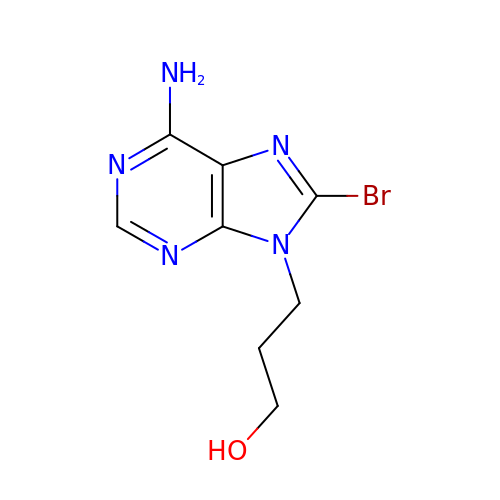3-(6-azanyl-8-bromanyl-purin-9-yl)propan-1-ol | C8 H10 Br N5 O | MUZYIFHIQGFDMZ-UHFFFAOYSA-N>MSQDNNYSQGPVPISARKGGLALTFVMLGLTFFSASMWTGGALGTGLSFNDFFLAVLIGNLLLGIYTAFLGFIGSKTGLTTHLLARYSFGIKGSWLPSFLLGGTQVGWFGVGVAMFAIPVGKATGIDINLLIAVSGILMTITVFFGISALTVLSIIAVPAIAILGSYSVYLAIHDMGGLSTLMNVKPTQPLDFNLALAMVVGSFISAGTLTADFVRFGRNPKVAVVVAIIAFFLGNTLMFVFGAAGAASLGMADISDVMIAQGLLLPAIVVLGLNIWTTNDNALYASGLG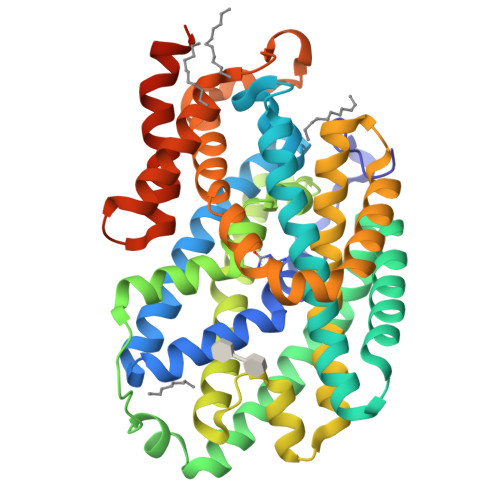FANITGLSSKKLSVINGIVGTVCALWLYNNFVGWLTFLSAAIPPVGGVIIADYLMNKARYNTFNIATMQSVNWVALLAVAIGIVAGHWLPGIVPVNAVLGGAISYAVLNPILNRRTARQAEISHAGSLEVLFQ[2x]>[6x]MAHHHHHHMIEWKTAKEYEDITYKKCNGVARIAFNRPEIRNAFRPKTTSELYDAFYDAYEDPSIGVVLLSGEGPSPKDGGWAFCSGGDQKARGHQGYVGEDGRHRLNILEVQRLIRFMPKVVIAVVPGWAVGGGHSLHVVCDLTLASKEHAIFKQTDADVTSFDGGYGSAYLAKMVGQ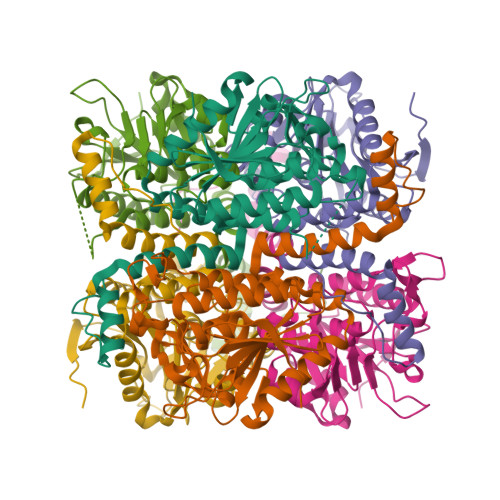KKAREIFFLGRNYSAQEAFEMGMVNKVVPHAELEDTAYEWAQEILAKSPTSIRMLKFAMNLTDDGMVGQQVFAGEATRLAYMTDEAKEGRNAFLEKRKPDFGEDQWIS N-benzyl-2-{4-[4-(4,5-dimethoxy-1H-indole-2-carbonyl)piperazine-1-carbonyl]piperidin-1-yl}-6-methylpyrimidine-4-carboxamide | C34 H39 N7 O5 | 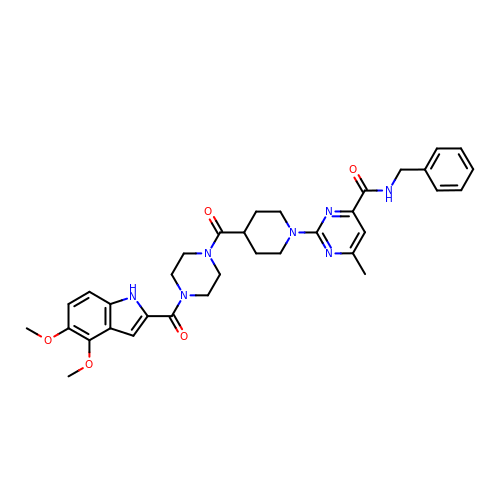PJHZEAWAAMNJHJ-UHFFFAOYSA-N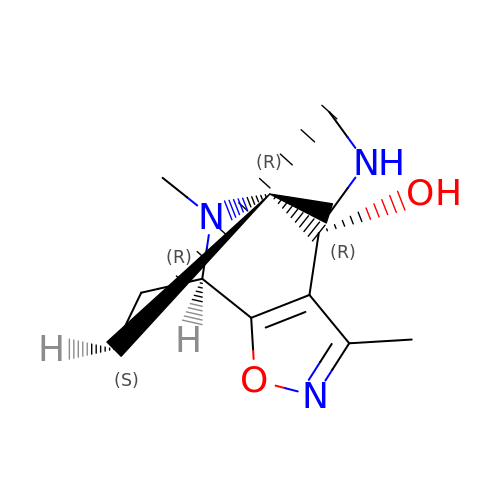(4R,4aR,7aS,9R)-3,10-dimethyl-5,6,7,7a,8,9-hexahydro-4H-4a,9-epiminopyrrolo[3',4':5,6]cyclohepta[1,2-d][1,2]oxazol-4-ol | C12 H17 N3 O2 | ORUIQGBPSJFGIC-MDSNHJATSA-N> GSTADKFRFFSMARDLLSWMESIIRQIETQERPRDVSSVELLMKYHQGINAEIETRSKNFSACLELGESLLQRQHQASEEIREKLQQVMSRRKEMNEKWEARWERLRMLLEVCQFSRDASVAEAWLIAQEP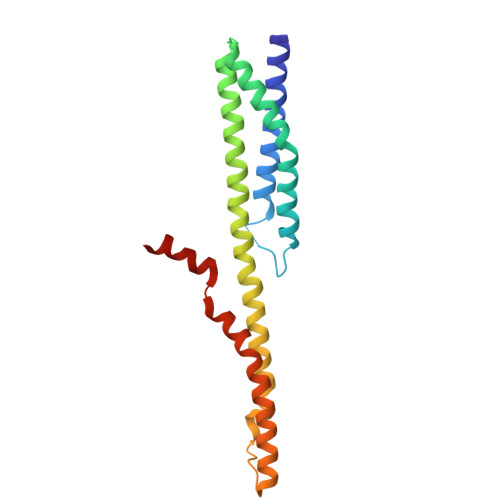YLASGDFGHTVDSVEKLIKRHEAFEKSTASWAERFAALEKPTTLELKERQIAER2-methoxy-4-(11-oxo-10,11-dihydro-5H-dibenzo[b,e][1,4]diazepin-3-yl)benzoic 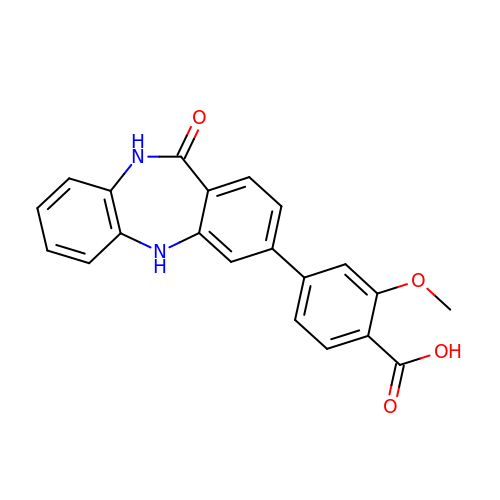acid | C21 H16 N2 O4 | OEIBPYXEHRSJOU-UHFFFAOYSA-N> MASWSHPQFEKGATTRILGVVQLDQRRLTDDLAVLAKSNFSSEYSDFACGRWEFCMLRNQSGKQEEQRVVVHETPA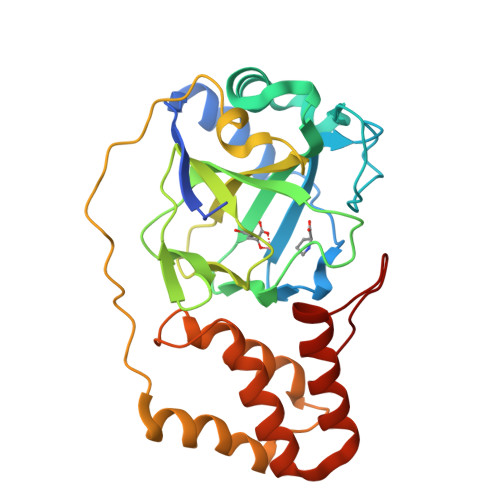LATPLGQSLPYLNELLDNHFDRDSIRYARIIRISENACIIPHRDYLELEGKFIRVHLVLDTNEKCSNTEENNIFHMGRGEIWFLDASLPHSAGCFSPTPRLHLVVDIEGTRSLEEVAINVEQPSARNATVDTRKEWTDETLESVLGFSEIISEANYREIVAILAKLHFFHKVHCVDMYGWLKEICRRRGEPALIEKANSLERFYLIDRAAGEVMTY>[3x]MNITKPFPLPTGYFGIPLGLAALSLAWFHLENLFPAARMVSDVLGIVASAVWILFILMYAYKLRYYFEEVRAEYHSPVRFSFIALIPITTMLVGDILYRWNPLIAEVLIWIGTIGQLLFSTLRVSELWQGGVFEQKSTHPSFYLPAVAANFTSASSLALLGYHDLGYLFFGAGMIAWIIFEPVLLQHLRISSLEPQFRATMGIVLAPAFVCVSAYLSINHG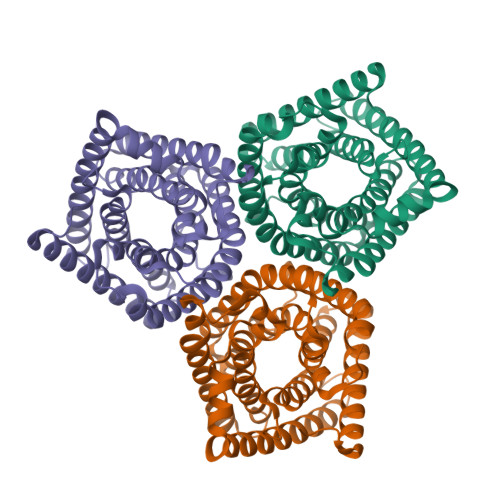EVDTLAKILWGYGFLQLFFLLRLFPWIVEKGLNIGLWAFSFGLASMANSATAFYHGNVLQGVSIFAFVFSNVMIGLLVLMTIYKLTKGQFFLK> GCCAG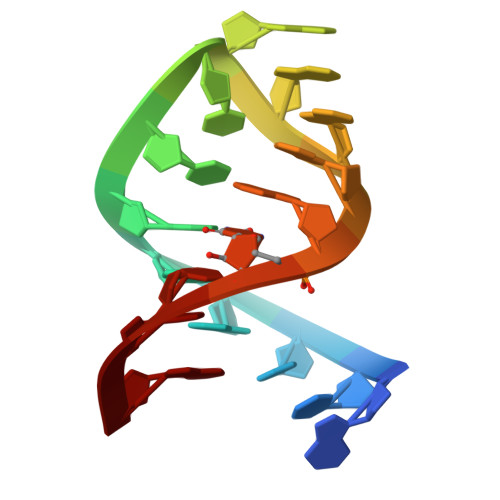ACUGAAGAUCUG>MRDHRKIGKQLDLYHMQEEAPGMVFWHNDGWTIFRELEVFVRSKLKEYQYQEVKGPFMMDRVLWEKTGHWDNYKDAMFTTSSENREYCIKPMNCPGHVQIFNQGLKSYRDLPLRMAEFGSCHRNEPSGSLHGLMRVRGFTQDDAHIFCTEEQIRDEVNGCIRLVYDMYSTFGFEKIVVKLSTRPEKRIGSDEMWDRAEADLAVALEENNIPFEYQLGEGAFYGPKIEFTLYDCLDRAWQCGTVQLDFSMPSRLSASYVGEDNERKVPVMIHRAILGSMERFIGILTEEFAGFFPTWLAPVQVVIMNITDSQSEYVNELTQKLSNAGIRVKADLRNEKIGFKIREHTLRRVPYMLVCGDKEVESGKVAVRTRRGKDLGSMDVNEVIEKLQQEIRSRSLKQLEELEHHHHHH[2x]

Here, we report that a critical glycine residue (Gly463) dominates the motion of threonyl-tRNA synthetase (ThrRS) and the sensitivity of the enzyme to antibiotics. The natural product Obafluorin (OB) is a potent inhibitor of bacterial threonyl-tRNA synthetase (ThrRS). Our previous work showed that OB covalently binds to ThrRS, forming an ester bond with a tyrosine residue in the catalytic center via the highly strained β-lactone ring, making OB the first covalent aaRS inhibitor with demonstrated crystal structures. The binding of OB induces a large conformational change in ThrRS.

In particular, Gly463 is adjacent to Tyr462, which is the residue covalently bound to OB, and Leu489 is located within 7 Å of the OB in the pocket. The results showed that 36j and OB increased the Tm of EcThrRS_L489M by 22.7 °C and 22.6 °C, respectively, suggesting that OB strongly binds to EcThrRS_L489M, similar to 36j. OB had a strong inhibitory effect on EcThrRS_L489M, with an IC50 value of 215 nM. Therefore, the mutation of Leu489 to a methionine does not confer resistance of EcThrRS to OB. An EcThrRS_L489M–OB complex structure was successfully obtained by cocrystallizing 300 μM EcThrRS_L489M protein with 600 μM OB. Because in the OB-binding conformation, the active pocket has a larger opening, we refer to this state as the “open state”. In short, the β-lactone ring of OB opens and forms an ester bond with Tyr462; the o-diphenol group forms coordination bonds with the ThrRS conserved Zn2+ ion; and the nitrobenzene group binds between Tyr313 and Arg363.>[6x]SRFESNPITLNDLSLGKPIAKGTNGVVYSAKVKD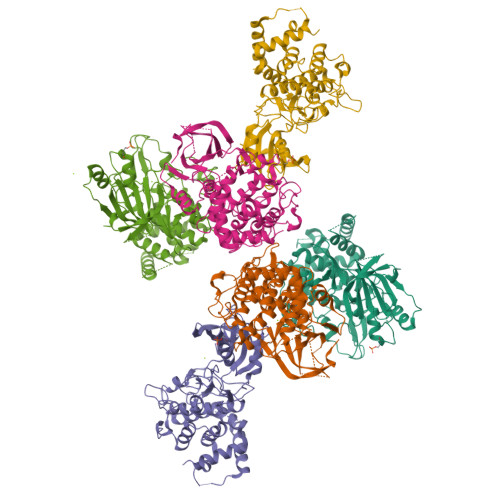DETDDNKYPFALKMMFNYDIQENSMEILKAMYRETVPARMYYSNHDLNNWEIELANRRKHLPPHPNIVAIFSVFTDLYPAALPPRLHPEGEGRNMSLFLLMKRYDCNLQSFLSTAPSTRTSLLLLAQLLEGVAHMTAHGIAHRDLKSDNLLLDTSEPESPILVISDFGCCLADKTNGLSLPYTSYEMDKGGNTALMAPEIICQKPGTFSVLNYSKADLWAVGAIAYEIFNCHNPFYGPSRLKNFNYKEGDLPKLPDEVPTVIQALVANLLKRNPNKRLDPEVAANVCQLFLWAPSTWLKPGLKVPTSGEILQWLLSLTTKVLCEGKINNKSFGAAFTRNWRRTYPEYLLISSFLCRAKLANVRNALHWIQENLPELD>[2x]SNADEEDANFMQRAFEMNDKVASDVMVDRTSMSVVDVDETIADALLLYLEEQYSRFPVTADNDKDKIIGYAYN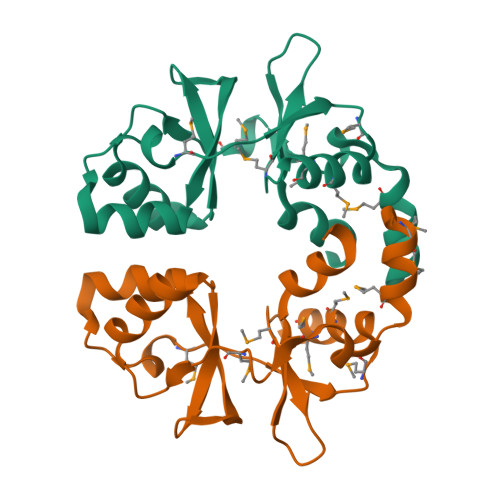YDIVRQARIDDKAKISTIMRDIVSVPENMKVPDVMEEMSAHRVPMAIVIDEYGGTSGIITDKDVYEELFGNLRDEQDDED>MAEKQYDFTHVPKRQGNSIKWGGLKEKELPMWIAEMDFRIAPEIMTSMEEKLKVAAFGYESVPAEYYKAVADWEEIEHRARPKEDWCVFASGVVPAISAMVRQFTSPGDQILVQEPVYNMFYSVIEGNGRRVISSDLIYENSKYSVNWADLEEKLATPSVRMMVFCNPHNPIGYAWSEEEVKRIAELCAKHQVLLISDEIHGDLVLTDEDITPAFTVDWDAKNWVVSLISPSKTFNLAALHAACAIIPNPDLRARAEESFFLAGIGEPNLLA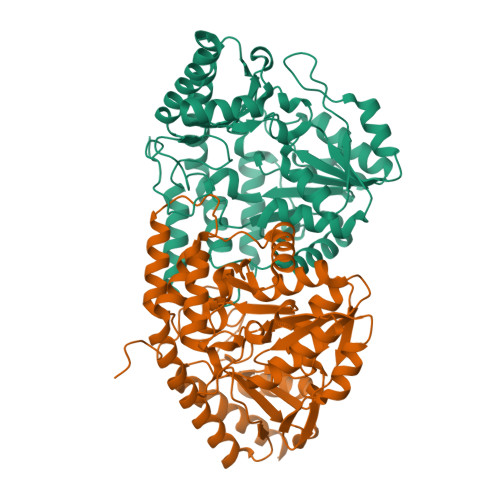IPAAIAAYEEGHNWLRELKQVLRDNFAYAREFLAKEVPEVKVLDSNASYLAWVDISALGMNAEDFCKYLREKTGLIISAGNGYRGNGHEFVRINLACPKELVIDGMQRLKQGVLNLNN[2x]> GSHMDQDSLSSSLKTCYKYLNQTSRSFAAVIQALDGEMRNAVCIFYLVLRALDTLEDDMTISVEKKVPLLHNFHSFLYQPDWRFMESKEKDRQVLEDFPTISLEFRNLAEKYQTVIADICRRMGIGMAEFLDKHVTSEQEWDKYCHYVAGLVGIGLSRLFSASEFEDPLVGEDTERANSMGLFLQKT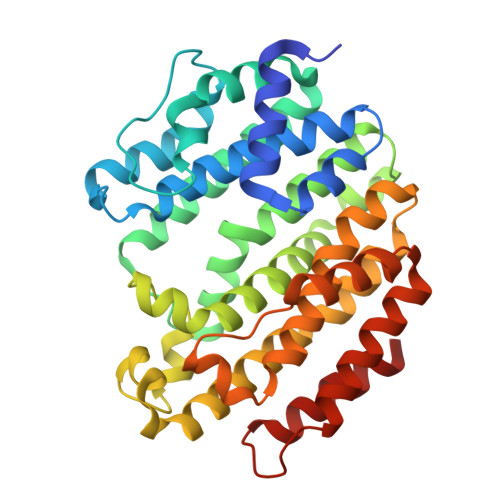NIIRDYLEDQQGGREFWPQEVWSRYVKKLGDFAKPENIDLAVQCLNELITNALHHIPDVITYLSRLRNQSVFNFCAIPQVMAIATLAACYNNQQVFKGAVKIRKGQAVTLMMDATNMPAVKAIIYQYMEEIYHRIPDSDPSSSKTRQIISTIRTQN>GHMPNIPPPFTAPYAPDDAEIAARLLPASHLSPPQEARIHRTATRLIEAIRKRDDRLGGVEDMLREFALSTKEGLALMVLAEALLRVPDARTADQFIEDKLGEGDFIHHETKSTAFLVNASAWALGLSARVIQPGETPDGTIGRLVKRLGAPAVRTATRQAMRLMGNHFVLGETIEQALERGKPRSGQKTRYSFDMLGEGARTAADARRYFDAYASAIETIGKAAGNHALPDRPGISVKLSALHPRFEAISRARVMVELVPQLLDLAQRAKAHDLNFTVDAEEADRLELSLDVIAATLADPSLKGWDGFGLAIQAYQKRASAVIDYVDALARAHDRKLMVRLVKGAYWDTEIKRAQERGLDGYPVFTRKAMTDLNYVACASKLLALRPRIFPQFATHNALTVATVLEMAEGSSGFEFQRLHGMGEALYEQLAKDHADIAYRTYAPVGSHRDLLAYLVRRLLENGANSSFVAQAADYRVPVPALLQRPADAIVRPQAAAHPRIPLPCDLFAPERRNSRGVEFGARTALDQLLTDVKAETGDLKPIADATPDQAHAAVAAARAGFAGWSRTPAGIRAAALEQAAHLLESRSAHFIALLQREGGKTLDDALSELREAADFCRYYAAQGRKLFGSETAMPGPTGESNALTMRGRGVFVAISPWNFPLAIFLGQVTAALMAGNSVVAKPAEQTPRIAREAVALLHEAGIPKSALYLVTGDGRIGAALTAHPDIA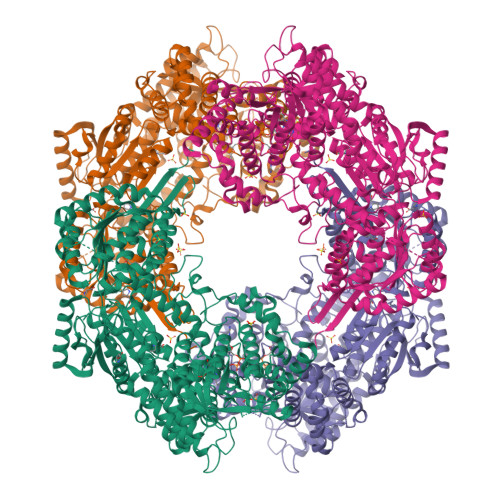GVVFTGSTEVARSINRALAAKDGPIVPLIAETGGINAMIADATALPEQVADDVVTSAFRSAGQRASALRLLFVQEDVADRMIEMVAGAARELKIGDPSDVATHVGPVIDVEAKQRLDAHIARMKTEARLHFAGPAPEGCFVAPHIFELTEAGQLTEEVFGPILHVVRYRPENLERVLRAIERTGYGLTLGVHSRIDDSIEAIIDRVQVGNIYVNRNMIGAVVGVQPFGGNGLSGTGPKAGGPHYLARFATEQTVTINTAAAGGNAALLAGEE[2x]>ATGTGKGVLGDTKSFTTTASGSSYQLKDTTRGNGVVTYTASNRQSIPGTILTDADNVWNDPAGVDAHTYAAKTYDYYKAKFGRNSIDGRGLQLRSTVHYGSRYNNAFWNGSQMTYGDGDGSTFIAFSGDPDVVGHELTHGVTEYTSNLEYYGESGALNEAFSDVIGNDIQRKNWLVGDDIYTPNIAGDALRSMSNPTLYDQPDHYSNLYTGSSDNGGVHTNSGIINKAYYLLAQGGTFHGVTVNGIGRDAAVQIYYSAFTNYLTSSSDFSNARAAV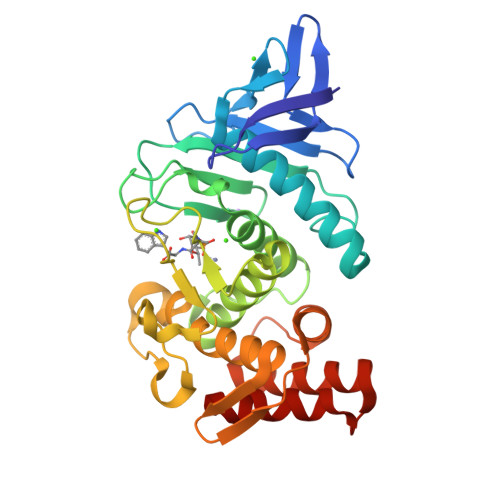IQAAKDQYGANSAEATAAAKSFDAVGVN[2x]> GSGKFGQQSGAIYVGNFRVVNRHLATHNDWANLVWEDSSRDLLVSSTTAQGCDTIARCNCQTGVYYCNSRRKHYPV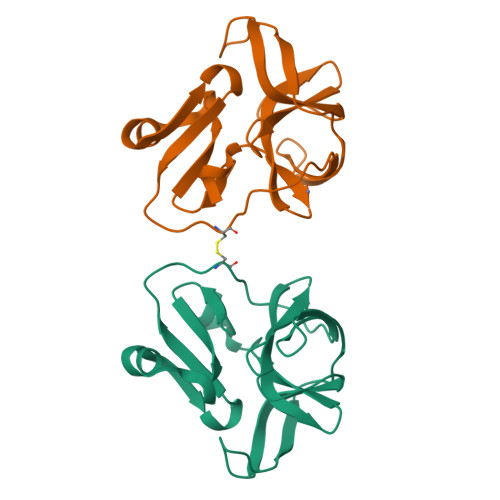SFSKPSLIYVEASEYYPARYQSHLMLAQGHSEPGDAGGILRCQHGVVGIVSTGGNGLVGFADVRDLLWLDEEAMEQ>GSDAQKQDWGNLKRYAEANKELVRKGKQKDRVVFMGNSITEGWVANDAAFFEDNGYVGRGIGGQTSSHFLLRFREDVIKLAPALVVINAGTNDIAENAGAYNEEYTFGNIVSMVELARANKIKVILTSVLPAAAFGWNPSVKDAPQKIMQLNA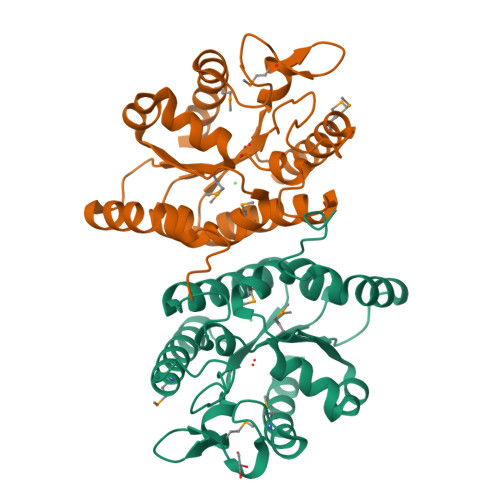RIRKYAQENKIPYVDYYSEMVEGDNKALNSSYTRDGVHPTLEGYKVMEALIKKAIDKVL[2x]>MLLNALASLGHKGIKTLRTFGRAGLMLFNALVGKPEFRKHAPLLVRQLYNVGVLSMLIIVVSGVFIGMVLGLQGYLVLTTYSAETSLGMLVALSLLRELGPVVAALLFAGRAGSALTAEIGLMRATEQLSSMEMMAVDPLRRVISPRFWAGVISLPLLTVIFVAVGIWGGSLVGVSWKGIDSGFFWSAMQNAVDWRMDLVNCLIKSVVFAITVTWISLFNGYDAIPTSAGISRATTRTVVHSSLAVLGLDFVLTALMFGN[2x];>[2x]MEQSVANLVDMRDVSFTRGNRCIFDNISLTVPRGKITAIMGPSGIGKTTLLRLIGGQIAPDHGEILFDGENIPAMSRSRLYTVRKRMSMLFQSGALFTDMNVFDNVAYPLREHTQLPAPLLHSTVMMKLEAVGLRGAAKLMPSELSGGMARRAALARAIALEPDLIMFDQPFVGQDPITMGVLVKLISELNSALGVTCVVVSHDVPEVLSIADHAWILADKKIVAHGSAQALQANPDPRVRQFLDGIADGPVPFRYPAGDYHADLLPGS;>[2x]MSESLSWMQTGDTLALSGELDQDVLLPLWEMREEAVKGITCIDLSRVSRVDTGGLALLLHLIDLAKKQGNNVTLQGVNDKVYTLAKLYNLPADVLPR;>MQTKKNEIWVGIFLLAALLAALFVCLKAANVTSIRTEPTYTLYATFDNIGGLKARSPVSIGGVVVGRVADITLDPKTYLPRVTLEIEQRYNHIPDTSSLSIRTSGLLGEQYLALNVGFEDPELGTAILKDGDTIQDTKSAMVLEDLIGQFLYGSKGDDNKNSGDAPAAAPGNNETTEPVGTTK[6x]

The IM MlaFEDB complex functions as an ABC transporter to translocate phospholipids between the IM and periplasm. This complex is composed of four components, namely the NBD protein MlaF, the TMD protein MlaE, the phospholipid-binding protein MlaD, and the auxiliary protein MlaB. MlaFEDB is assembled in a stoichiometry of 2:2:6:2 (MlaF:MlaE:MlaD:MlaB). MlaD forms a hexameric disc-shaped ring on top of MlaE, with a central pore lined by hydrophobic residues and has been shown to contain phospholipids.

For cryo-EM studies, the purified MlaFEDB complex with the E170Q mutation (MlaFEQEDB) was incubated with 2 mM ATP-Mg2+ prior to the preparation of cryo-EM specimen. Image processing generated cryo-EM maps of the MlaFEQEDB complex in different conformations (EQtall and EQclose) at resolutions of 4.3 and 3.7 Å, respectively. In contrast, the ATP-binding sites in EQtall structure are more open, suggesting that the two MlaF subunits do not adopt an ATP-bound conformation with tightly dimerized NBDs. The structure of EQtall showed a major conformational rearrangement of MlaD. The hexametric ring of the MCE domain in MlaD is lifted, increasing the height of the entire complex (left). The ring of MCE domains also twisted clockwise, when viewed from the periplasmic side, by ~15°. The MlaE, MlaF and MlaB are essentially identical to those in the structure of nucleotide-free complex. The lift-up movement of MCE domain of MlaD leads to an extension of the central hydrophobic cavity formed by MlaE and MlaD to the periplasmic side, which may facilitate the movement of phospholipids to and/or from the periplasm. The density traces of a phospholipid tail was observed in the central cavity, suggesting the EQtall is in a transit state of lipid translocation. The structure of EQtall suggests that MlaD lift-up may facilitate the transport of the phospholipids bound inside the central cavity, which may help to move the bound phospholipids upwards to reach MlaD in the periplasm.The tip of each stereocilium is linked to its tallest neighbor by a ‘tip link' filament essential for hair-cell mechanotransduction. Immature tip links are likely formed by homotetrameric protocadherin-15 (PCDH15) proteins, while mature tip links are made of cadherin-23 (CDH23) and PCDH15 heterotetramers. CDH23 and PCDH15 are unusual members of the family that feature 27 and 11 EC repeats, respectively. Here we present the X-ray crystal structures of repeats EC8–10 and EC9–10 refined at 2.8 and 3.35 Å resolution, respectively, which show an EC9–10 calcium-free linker that alters the linear arrangement of PCDH15's EC repeats.

To understand the role of non-canonical tip-link EC repeats, the human protocadherin-15 EC8–10 (PCDH15 EC8–10) and the mouse EC9–10 (mmPcdh15 EC9–10) fragments were refolded from inclusion bodies produced in Escherichia coli and used for crystallization and structural determination. The structure for mouse Pcdh15 EC9–10 (3.35 Å) contained 228 residues starting from Met 898 to Glu 1,125 (in the most complete protomer of the four found in the asymmetric unit). A structure of mouse Pcdh15 EC9–10 (without EC8), crystalized in a different condition and space group, shows the same unique features. This suggests that the EC9–10 interface is robust and that the observed features are not a crystallographic artifact (Supplementary Discussion). Sequence analysis indicates the absence of canonical calcium-binding motifs in the PCDH15 EC9–10 linker across different species. Consistently, the PCDH15 EC9–10 region shows a calcium-free linker that is bent (∼90°) and breaks the linear arrangement of EC repeats. In addition, the PCDH15 EC9–10 linker has structural features not observed in DNcad, Tcad or any other cadherin structures. A unique EC9–10 310 helix is located in the middle of the EC9–10 linker (His 1,007–Ile 1,011; blue arrow in Fig. 1d,e), and an atypical EC10 FG-α loop (Leu 1,091–Asn 1,105) form an EC9–10 interface that stabilizes the observed bent conformation of the linker. In addition, EC9 and EC10 have unusual and unique structural features involved in bending, namely an EC9–10 310 helix and an EC10 FG-α loop that form part of an interface that keeps EC9 stuck to EC10. Also, unbending was not observed and the end-to-end angle and distance were stable throughout both simulations. This suggests that the EC9–10 repeats are bent in solution, spontaneously and occasionally transitioning between two very similar bent states. Overall, the data presented here strongly suggest that the bent, calcium-free linker in PCDH15 EC9–10 plays a relevant mechanical role in hair-cell transduction.

>[4x]MNDYPPVFSKRIYKGMVAPDAVKGTPITTVYAEDADPPGMPASRVRYRVDDVQFPYPASIFDVEEDSGRVVTRVNLNEEPTTIFKLVVVAFDDGEPVMSSSATVRILVLHPGEIPRFTQEEYRPPPVSELAARGTVVGVISAAAINQSIVYSIVAGNEEDKFGINNVTGVIYVNSPLDYETRTSYVLRVQADSLEVVLANLRVPSKSNTAKVYIEIQDENDHPPVFLEHHHHHH>ADKNPGSENMTNTIGPHDRGGSSPIYNILNSYLTAYNGSHHLYDRMSFLCLSSQNTLNGACPSSDAPGTATIDGETNITLQFTEKRSLIKRELQIKGYKQFLFKNANCPSKLALNSSHFQCNREQASGATLSLYIPAGELNKLPFGGVWNAVLKLNVKRRYDTTYGTYTINITVNLTDKGNIQIWLPQFKSNARVDLNLRPTGGGTYIGRNSVDMCFYDGYSTNSSSLEIRFQDDNSKSDGKFYLKKINDDSKELVYTLSLLLAGKNLTPTNGQ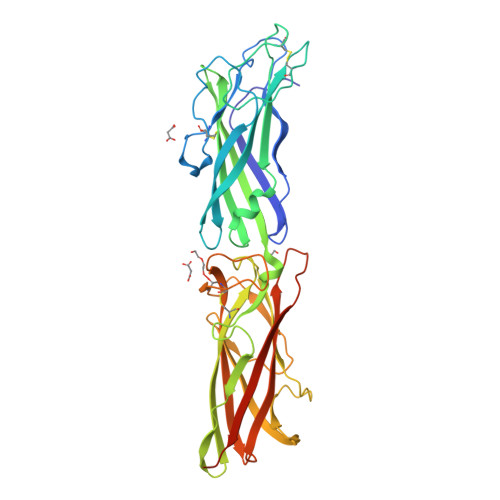ALNINTASLETNWNRITAVTMPEISVPVLCWPGRLQLDAKVKNPEAGQYMGNIKITFTPSSQTLDNKQVEKNITVTASVDPVIDLLQLEHHHHHH[2x]> MPRSTWKGPYVAVSLLQEVVALARKHPNWWNKGRYIGQKAPEVINTY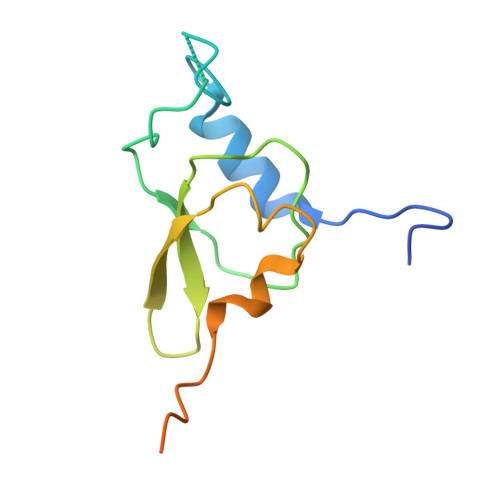SRASVILPDFIACRFGVHNGKSFVGMEVQEAMVGHRLGEFAPTKATVQHKAKEVNTQKKKINPKTGKAA N-[6-(1,2,3,4-tetrahydroacridin-9-ylamino)hexyl]pyridine-3-carboxamide 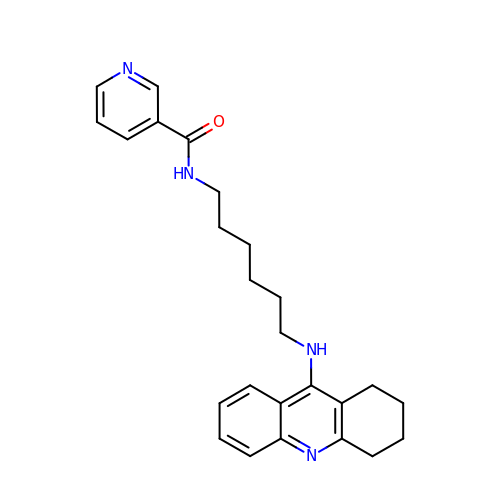| C25 H30 N4 O | QMTDQDYAGOQABA-UHFFFAOYSA-N> V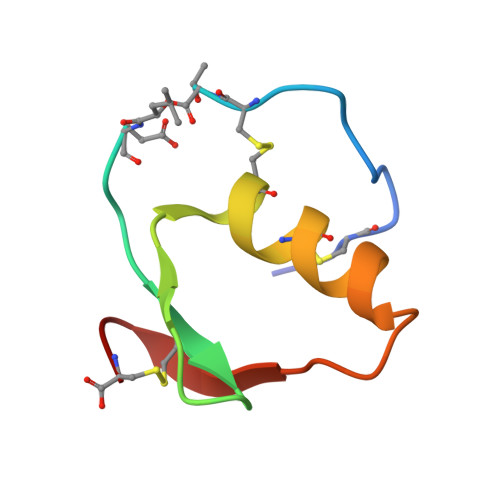DCSEYPKPACTXEYRPLCGSDNKTYGNKCNFCNAVVESNGTLTLSHFGKC(R)-N-(7-(4-((4'-chlorobiphenyl-2-yl)methyl)piperazin-1-yl)quinazolin-4-yl)-4-(4-(dimethylamino)-1-(phenylthio)butan-2-ylamino)-3-nitrobenzenesulfonamide 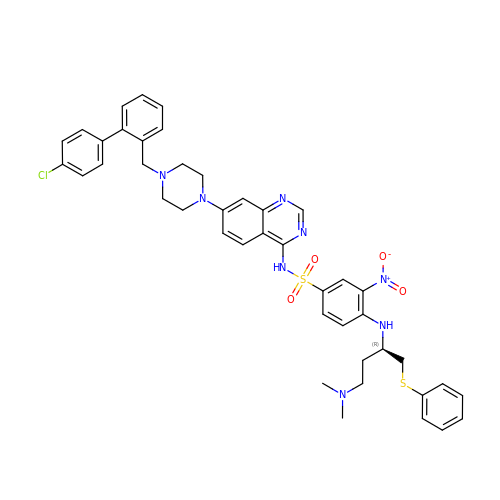| C43 H45 Cl N8 O4 S2 | LLJSSTLCMHGPSB-UUWRZZSWSA-N> GSSHHHHHHSSGLVPRGSMSTSWSDRLQNAADMPANMDKHALKKYRREAYHRVFVNRSLAMEKIKCFGFNMDYTLAVYKSPEYESLGFELTVERLVSIGYPQELLSFAYDSTFPTRGLVFDTLYGNLLKVDAYGNLLVCAHGFNFIRGPETREQYPNKFIQRDDTERFYILNTLFNLPETYLLACLVDFFTNCPRYTSCETGFKDGDLFMSYRSMFQDVRDAVDWVHYKGSLKEKTVENLEKYVVKDGKLPLLLSRMKEVGKVFLATNSDYKYTDKIMTYLFDFPHGPKPGSSHRPWQSYFDLILVDARKPLFFGEGTVLRQVDTKT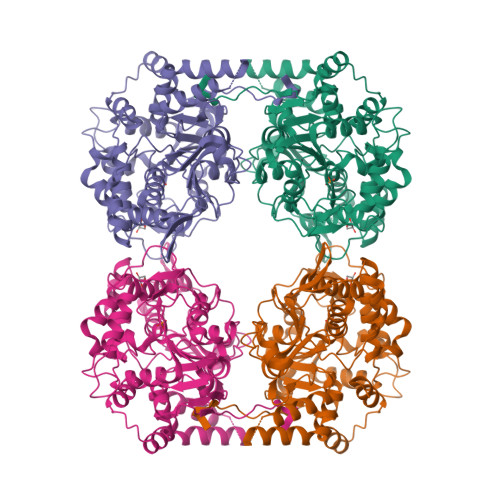GKLKIGTYTGPLQHGIVYSGGSSDTICDLLGAKGKDILYIGDHIFGDILQSKKRQGWRTFLVIPELAQELHVWTDKSSLFEELQSLDIFLAELYKHLDSSSNERPDISSIQRRIKKVTHDMDMCYGMMGSLFRSGSRQTLFASQVMRYADLYAASFINLLYYPFSYLFRAAHVLMPHESTVEHTHVDINEMESPLATRNRTSVDFKDTDYKRHQLTRSISEIKPPNL> MFSAGHKIKGTVVLMPKNELEVNPDGSAVDNLNAFLGRSVSLQLISATKADAHGKGKVGKDTFLEGINTSLPTLGAGESAFNIHFEWDGSMGIPGAFYIKNYMQVEFFLKSLTLEAISNQGTIRFVCNSWVYNTKLYKSVRIFFANHTYVPSETPAPLVSYREEELKSLRGNGTGERKEYDRIYDYDVYNDLGNPDKSEKLARPVLGGSSTFPYPRRGRTGRGPTVTDPNTEKQGEVFYVPRDENLGHLKSKDALEIGTKSLSQIVQPAFESAFDLKSTPIEFHSFQDVHDLYEGGIKLPRDVISTIIPLPVIKELYRTDGQHILKFPQPHVVQVSQSAWMTDEEFAREMIAGVNPCVIRGLEEFPPKSNLDPAIYGDQSSKITADSLDLDGYTMDEALGSRRLFMLDYHDIFMPYVRQINQLNSAKTYATRTILFLREDGTLKPVAIELSLPHSAGDLSAAVSQVVLPAKEGVESTIWLLAKAYVIVNDSCYHQLMSHWLNTHAAMEPFVIATHRHLSVLHPI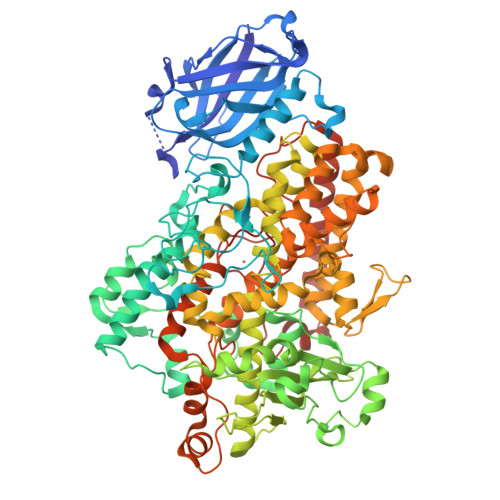YKLLTPHYRNNMNINALARQSLINANGIIETTFLPSKYSVEMSSAVYKNWVFTDQALPADLIKRGVAIKDPSTPHGVRLLIEDYPYAADGLEIWAAIKTWVQEYVPLYYARDDDVKNDSELQHWWKEAVEKGHGDLKDKPWWPKLQTLEDLVEVCLIIIWIASALHAAVHFGQYPYGGLIMNRPTASRRLLPEKGTPEYEEMINNHEKAYLRTITSKLPTLISLSVIEILSTHASDEVYLGQRDNPHWTSDSKALQAFQKFGNKLKEIEEKLVRRNNDPSLQGNRLGPVQLPYTLLYPSSEEGLTFRGIPNSISI> GHMQETQAVEAGEKTVEQFVQALNKGDYNKAAEMTSKKAANKSALSEKEILDKYQNIYGAADVKGLQISNLKVDKKDDSTYSFSYKAKMNTSLGELKDLSYKGTLDRNDGQTTINWQPNLVFPEMEGNDKVSLTTQEAARGNIIDRNGEPLATTGKLKQLGVVPSKLGDGGEKTANIKAIASSFDLTEDAINQAISQSWVQPDYFVPLKIIDGATPELPAGATIQEVDGRYYP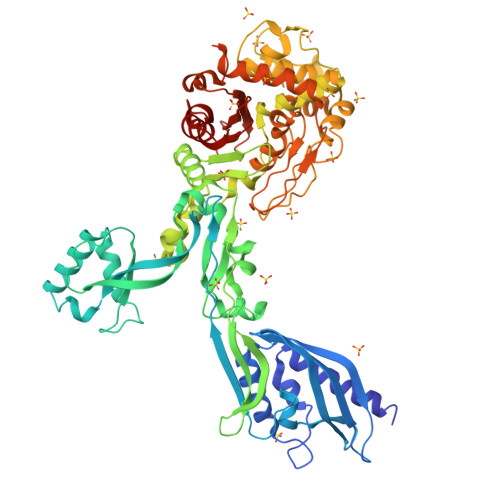LGEAAAQLIGYVGDITAEDIDKNPELSSNGKIGRSGLEMAFDKDLRGTTGGKLSITDADGVEKKVLIEHEVQNGKDIKLTIDAKAQKTAFDSLGGKAGSTVATTPKTGDLLALASSPSYDPNKMTNGISQEDYKAYEENPEQPFISRFATGYAPGSTFKMITAAIGLDNGTIDPNEVLTINGLKWQKDSSWGSYQVTRVSDVSQVDLKTALIYSDNIYMAQETLKMGEKKFRTGLDKFIFGEDLDLPISMNPAQISNEDSFNSDILLADTGYGQGELLINPIQQAAMYSVFANNGTLVYPKLIADKETKDKKNVIGETAVQTIVPDLREVVQDVNGTAHSLSALGIPLAAKTGTAEIKEKQDVKGKENSFLFAFNPDNQGYMMVSMLENKEDDDSATKRASELLQYLNQNYQ2-amino-N'-{3-[(E)-{2-[(2S)-2-amino-3-(1H-indol-3-yl)propanoyl]hydrazinylidene}methyl]benzylidene}-3-(1H-indol-2-yl)propanehydrazide 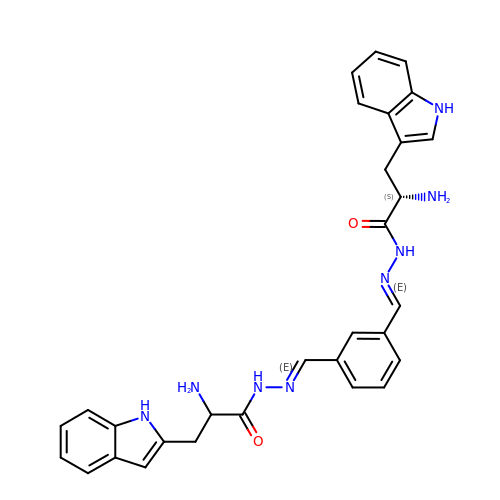(non-preferred name) | C30 H30 N8 O2 | ZUYUCFMTHKDHJX-JQHDDIPESA-N>HMGIEYRSLHTSQLTLSEKEALYDLLIEGFEGDFSHDDFAHTLGGMHVMAFDQQKLVGHVAIIQRHMALDNTPISVGYVEAMVVEQSYRRQGIGRQLMLQTNKIIASCYQLGLLSASDDGQKLYHSVGWQIWKGKLFELKQGSYIRSIEEEGGVMGWKADGEVDFTASLYCDFRGGDQW[2x]

However, a newly developed aminoglycoside antibiotic, plazomicin (marketed as Zemdri), was approved for clinical use by the U.S. Food and Drug Administration (FDA) in 2018; and since then, sister agencies in other countries have also approved its use. Like other aminoglycosides, plazomicin binds to the 16S rRNA at the aminoacyl-tRNA site (A-site) of the 30S ribosomal subunit, interfering with protein translation. Chemically, plazomicin is derived from sisomicin, an aminoglycoside that closely resembles gentamicin, with synthetic modifications incorporated at the N1 and N6′ positions of the antibiotic. The N1 position is extended by appending a hydroxy-aminobutyric acid (HABA) substituent, and the N6′ is modified through the addition of a hydroxyethyl (HE) substituent.

The high-resolution crystal structure of acetylated-plazomicin and CoA bound to AAC(2′)-Ia from Providencia stuartii was determined at 2.0 Å. Crystals of AAC(2′)-Ia were grown in the presence of the substrates plazomicin and acetyl-CoA. However, discovery maps unequivocally identified the enzymatically modified plazomicin and CoA in the active site in each unit of the dimeric structure, indicating that the acetylation reaction had occurred during crystallization and that the product bound state of the enzyme was captured. The AAC(2′)-Ia plazomicin binding pocket primarily wraps around the central and prime rings of the aminoglycoside, while the double-prime ring is relatively solvent-exposed. The pattern of hydrogen bonds between AAC(2′)-Ia and acetylated-plazomicin reveals that the majority of interactions occur at the central ring and the prime ring, the latter being the site of 2′-aminoglycoside modification. The Ser114 interacts with the 2′-amine, while residues Ala80 and Met81 interact with the oxygen of the 2′-acetyl modification. The N1 HABA tail extends away from the central ring in a solvent-exposed region, though the N1 secondary amine moiety forms hydrogen bonds with Glu149 and Asp176. The N6′ HE extension sits in a crescent-shaped tunnel of the enzyme and forms a hydrogen bond with residues Asp32 and 37. The structure of the plazomicin enzyme complex shows the reason for this, i.e., the aminoglycoside binding pocket of AAC(2′)-Ia can accommodate both the HABA and HE extensions, while the enzyme remains perfectly poised to modify one of the functional groups on the antibiotic. Modeling of the inactivated plazomicin into the ribosomal A-site reveals that the carbonyl group of the additional acetyl moiety would inevitably cause steric clashes with O6 and/or N7 of G1491.>[4x]MSSSVPTVKLFIGGKFVESKSDKWIDIHNPATNEVIGRVPQATKAEMDAAIASCKRAFPAWADTSVLSRQQVLLRYQQLIKENLKEIAKLITLEQGKTLADAEGDVFRGLQVVEHACSVTSLMMGETMPSITKDMDLYSYRLPLGVCAGIAPFNFPAMIPLWMFPMAMVCGNTFLMKPSERVPGATMLLAKLLQDSGAPDGTLNIIHGQHEAVNFICDHPDIKAISFVGSNKAGEYIFERGSRHGKRVQANMGAKNHGVVMPDANKENTLNQLVGAAFGAAGQRCMALSTAVLVGEAKKWLPELVEHAKNLRVNAGDQPGADLGPLITPQAKERVCNLIDSGTKEGASILLDGRKIKVKGYENGNFVGPTIISNVKPNMTCYKEEIFGPVLVVLETETLDEAIQIVNNNPYGNRTAIFTTNGATARKYAHLVDVGQVGVNVPIPVPLPMFSFT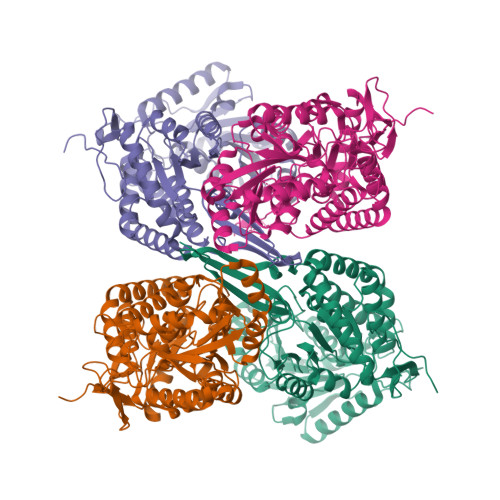GSRSSFRGDTNFYGKQGIQFYTQLKTITSQWKEEDATLSSPAVVMPTMGRENLYFQ>[2x]MPFTIDSARGIFPNTLAADVVPATIARFSQLNAEDQLALIWFAYLEMGKTLTIAAPGAASMQLAENALKEIQAMGPLQQTQAMCDLANRADTPLCRTYASWSPNIKLGFWYRLGELMEQGFVAPIPAGYQLSANANAVLATIQGLESGQQITVLRNAVVDMGFTAGKDGKRIAEPVVPPQDTASRTKVSIEGVTNATVLNYM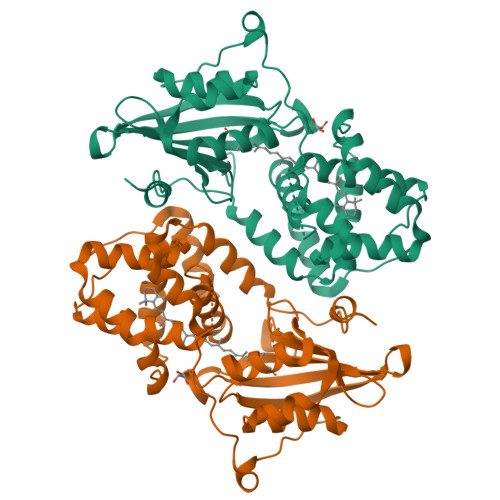DNLNANDFDTLIELFTSDGALQPPFQRPIVGKENVLRFFREECQNLKLIPERGVTEPAEDGFTQIKVTGKVQTPWFGGNVGMNIAWRFLLNPEGKIFFVAIDLLASPKELLNFAVHHHHHH> MCFSPKIKTPKMDTNQIRAVEPAPLT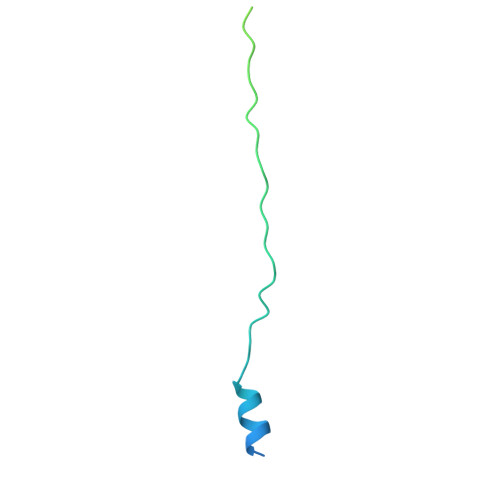QEVSSVEFGGSSDETDTEGTEVSGRKGLKVERDDSVAKSKASGNGSARMKSSIRKSAFGGKK>[6x]MYEEFPDVITFQSYVEQSNGEGGKTYKWVDEFTAAAHVQPISQEEYYKAQQLQTPIGYNIYTPYDDRIDKKMRVIYRGKIVTFIGDPVDLSGLQEITRIKGKEDGAYVG;>[12x]MADIYPLGKTHTEELNEIIVESAKEIAEPDTTMIQKLIDEHNPEPLLKGVRYYMCENDIEKKRRTYYDAAGQQLVDDTKTNNRTSHAWHKLFVDQKTQYLVGEPVTFTSDNKTLLEYVNELADDDFDDILNETVKNMSNKGIEYWHPFVDEEGEFDYVIFPAEEMIVVYKDNTRRDILFALRYYSYKGIMGEETQKAELYTDTHVYYYEKIDGVYQMDYSYGENNPRPHMTKGGQAIGWGRVPIIPFKNNEEMVSDLKFYKDLIDNYDSITSSTMDSFSDFQQIVYVLKNYDGENPKEFTANLRYHSVIKVSGDGGVDTLRAEIPVDSAAKELERIQDELYKSAQAVDNSPETIGGGATGPALENLYALLDLKANMAERKIRAGLRLFFWFFAEYLRNTGKGDFNPDKELTMTFTRTRIQNDSEIVQSLVQGVTGGIMSKETAVARNPFVQDPEEELARIEEEMNQYAEMQGNLLDDEGGDDDLEEDDPNAGAAESGGAGQVS;>MDIQRVKRLLSITNDKHDEYLTEMVPLLVEFAKDECHNPFIDKDGNESIPSGVLIFVAKAAQFYMTNAGLTGRSMDTVSYNFATEIPSTILKKLNPYRKMAR[12x]

Many double-stranded DNA (dsDNA) viruses have a specialized portal complex at one 5-fold vertex of their icosahedral capsid through which dsDNA enters and exits the virion. Sealing of the portal channel is achieved by binding head completion proteins to assemble a complex named connector in tailed prokaryotic viruses, which consists of stacked cyclical oligomers creating a channel for DNA traffic. In bacteriophage SPP1, the gp15 and gp16 head completion proteins bind sequentially to the dodecameric portal protein gp6 after DNA packaging. The gp15 adaptor protein extends the portal tunnel that is fastened afterwards by binding the gp16 stopper protein.

Here we report a cryoEM structure of the 902 kDa bacteriophage SPP1 connector in the post-DNA packaging state at a resolution of 2.7 Å. We have found that the connector comprises 12 subunits of both gp6 and gp15, but only 6 copies of gp16 in contrast to previous reports. Gp6 encompasses four major domains: the crown, wing, stem, and clip. In the connector gp6, Pro296 is shifted upwards by 7 Å bringing helix α4 to a more horizontal orientation closer to the gp6 β-hairpin of subunit i + 2. These changes in the clip domains of the connector gp6 lead to formation of pockets where the C-termini of gp15 bind to the portal oligomer. Gp15 interacts with the gp6 oligomer mostly via insertion of its C-terminus into the gp6 clip pocket. The most dramatic conformational change takes place by folding of loop α2-α3 into the β1-β2 hairpin that forms the gp15 24-stranded intermolecular β-barrel. The gp15 β1-β2 hairpins of neighbour subunits form an intersubunit 24-stranded β-barrel distal from the portal that outlines the 34 Å-wide central tunnel of gp15. Each gp16 subunit makes contacts with four gp15 subunits. A second type of interactions between gp16 and gp15 takes place by insertion of the gp16 N-terminus from chain k + 1 in a crease between the gp15 β-barrel and loops α2-β1 of gp15 chains j and j + 1, respectively. This network of interactions establishes the transition of 12 to 6-fold symmetry within the connector. The tunnel helices form a constriction in the portal channel with a diameter of ~12 Å between side chains of opposite gp16 Gln51 residues.> MAPLRKTAVLKLYVAGNTPNSVRALKTLNNILEKEFKGVYALKVIDVLKNPQ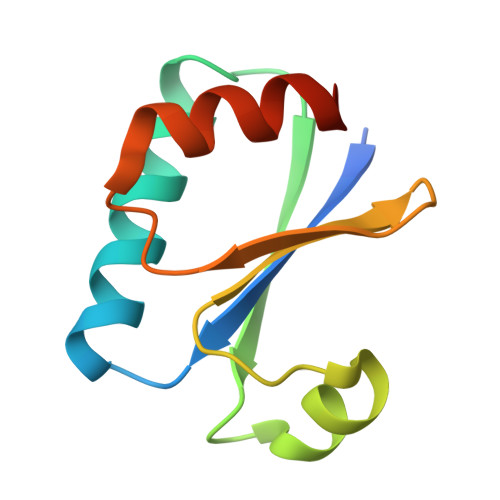LAEEDKILATPTLAKVLPPPVRRIIGDLSNREKVLIALRLLAEEIGD>VNFPNIPAEGVQFRLRARDTGYVIYSRTENPPLVWQYNGPPYDDQLFTLIYGTGPRKNLYAIKSVPNGRV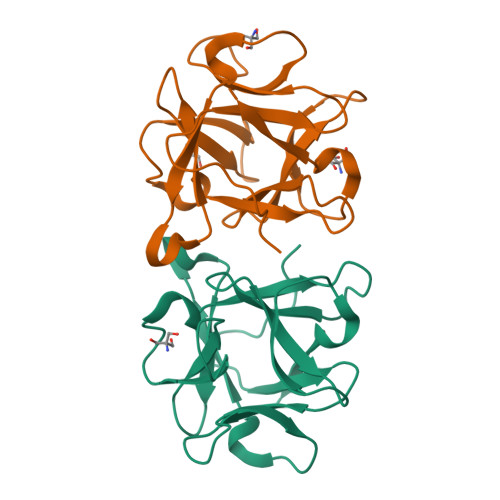LFSRTSASPYVGNIAGDGTYNDNWFQFIQDDNDPNSFRIYNLASDTVLYSRTTADPKFGNFTGAKYDDQLWHFELV[2x]> IEALVPAWDSDIIFKCLCYFHTLYPGLIPLETFPPATIFNFKQKIISILEDKKAVLRGEPIKGPLPICCSKENYRRHLQRTTLLPVFMWYHPTPKTLSDTMQTMKQLAIKGSVGASHWLLVIVDIQARRLVYFDSLYNYVMPPENMKKELQSFAQQLDQVYPAYDSKKFS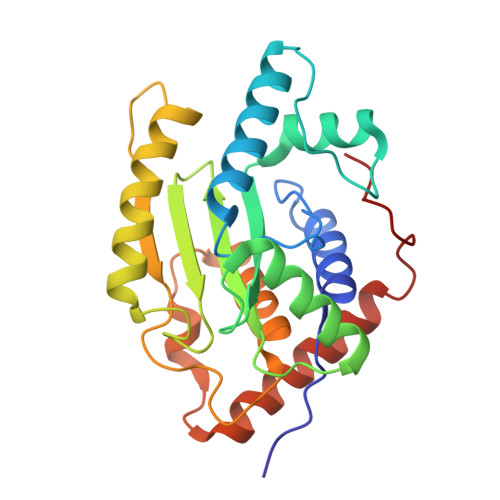VKIAAKEVIQRGSGSSCGAWCCQFLHWYLKDPLTDALNDLPVDSVERHENLASFVQACEAAVQDLPELSWPEA;> GPRRQTIEALVPAWDSDIIFKCLCYFHTLYPGLIPLETFPPATIFNFKQKIISILEDKKAVLRGEPIKGPLPICCSKENYRRHLQRTTLLPVFMWYHPTPKTLSDTMQTMKQLAIKGSVGASHWLLVIVDIQARRLVYFDSLYNYVMPPENMKKELQSFAQQLDQVYPAYDSKKFSVKIAAKEVIQRGSGSSCGAWCCQFLHWYLKDPLTDALNDLPVDSVERHENLASFVQACEAAVQDLPELSWPEA> GME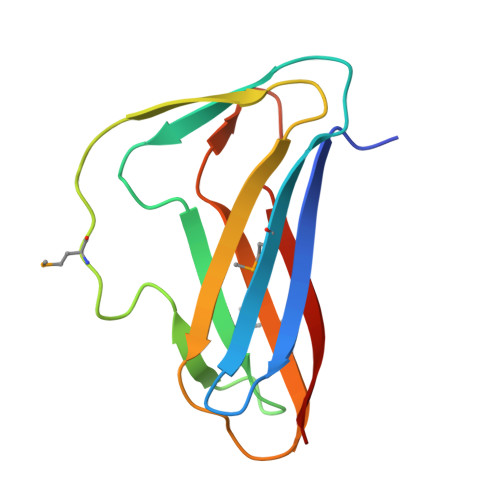NQEVVLSIDAIQEPEQIKFNMSLKNQSERAIEFQFSTGQKFELVVYDSEHKERYRYSKEKMFTQAFQNLTLESGETYDFSDVWKEVPEPGTYEVKVTFKGRAENLKQVQAVQQFEVK>MGHHHHHHHHHHSSGHIEGRHMSVVELEDGVYESTAVIDNGSFGTRTIRFETGRLAQQAAGSAVAYLDDETMLLSATTASKNPKDHFDFFPLTVDVEERMYAAGRIPGSFFRREGRPSTDAILTCRLIDRPLRPSFVDGLRNEIQVVVTVMSLDPKDLYDVLAINAASMSTQLAGLPFSGPVGGARIALIDGTWVAFPTVEQLERAVFDMVVAGRIVGDGDSADVAIMMVEAEATENVVELVAGGAQAPTEAVVAEGLEAAKPFIKALCAAQQELADRAAKPAGEYPVFPDYEADVYDAVASVATEALAEALTIAGKTERNDRTDEIKVEVLERLAEPYAGREKEIGAAFRSLTKKLVRQRILTDHFRIDGRGITDIRALSAEVAVIPRAHGSALFERGETQILGVTTLDMIKMAQQIDSLGPENTKRYMHHYNFPPYSTGETGRVGSPKRREIGHGALAERALVPVLPSIEEFPYAIRQVSEALGSNGSTSMGSVCASTLALLNAGVPLKAPVAGIAMGLVSDDVDVDGKVEKRYVALTDILGAEDAFGDMDFKVAGTK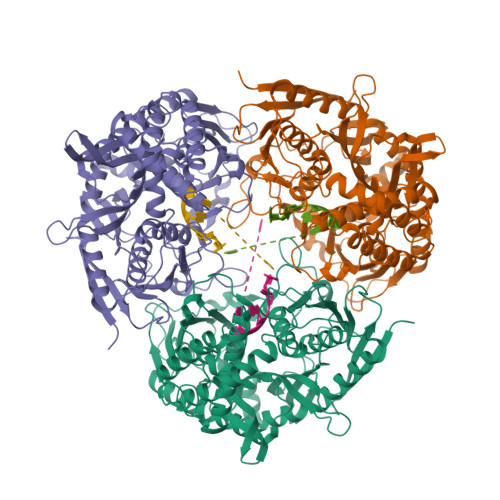DFVTALQLDTKLDGIPSQVLAGALSQAKDARLTILDVMAEAIDRPDEMSPYAPRITTIKVPVDKIGEVIGPKGKMINSITEETGAQISIEDDGTVFVGAADGLSAQAAIDKINAIANPQLPKVGERFLGTVVKTTDFGAFVSLLPGRDGLVHISKLGKGKRIAKVEDVVKVGDKLRVEIADIDNRGKISLVLVAEESAESAESAGDKGAEKAEGAAADVTPAEA[3x]> SHLDKVQPVIKNSDMSVEMQK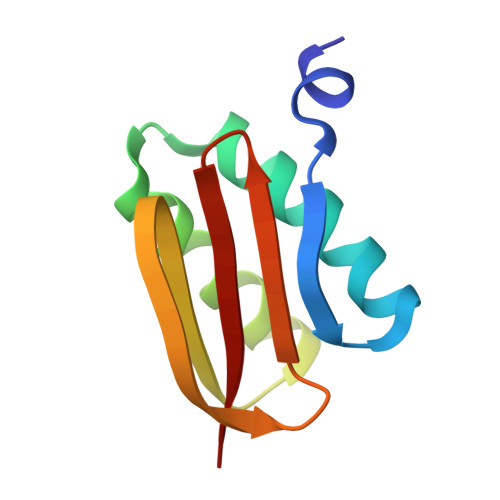EVEEVAKKAIDYCNTDKEIATFIKDDFRSRYHGTWHCIVGRNFGSFVTFERSYYIYLYVGQLAILLFKTG>[5x]MYFFSVDPRNGASKSGDVCGSCCCESISARPGEVNGVMVSYAAWSAPLRGHGLTNKTTFEIDGVSVTPPKVSNAFGRTKVGVVFEGTLSDLFPNPEGEQVEYEISELNGPSNGVVELGANGAFTYTPGALFTGVDRFWFSINGNIGEYVISVDPTTSELPQPPFTTPVYVPAARRSVDPRTHVLKFVLGVSPAAIPGDVYRLTVRQVAIDCDGNEFVHISCYDISIGSCG;>METKLTYGNRVTLPEFAKYIVAPAFHEIEGRAIPVTGVDDDASGTQATKLPFVLVGLRQGDTSGPATIAGNSTINLRDDFIVEFNMKKERYRDRKGGETPFFSYYDYESIRDRLFNSMIEFSGEHGITFEFVSLDISTEGDVVYIEFRFRQNYEWCETVREADTTIEAGRFSINLQGC[2x];>MACNKQNGVKNILITFTDCDTQEVIGPISHEQPDDTLPTYKNCAWTNTALTNGYVQRSASNATMTLPVVRDLRVPLAFYQGCAQVDVQVEKFDGTVMTLTEGAVVEPEESDGRSVTMNIVASEIDELLPPGSLAAA[4x];>MAQDALSDGFVRLCIDPSLNFFGEGCKILVEGQMTDDGSATPDAVTCVTSELDIIERFGQGSVLTESLRKVFCTCKSGVSVYALPREDAAAGVKAVYTLTIAGPATTDGRVQLYMGEAEYAVDIGVDAGDTATDIAAAIVAAISPDFPYAATAAAGVITLTARNAGTIGNHLSVIYTNLGSCTSVTPEGVTVTFAQTTAGSVNPTPNDYATVVNECCFAVYVLSSDDTDWQENLRDWIRSAWDCSKPQCFGHGYVFNKGTLGQVLADGDNSAELSRLALPTTYPVLPYLTNAAYGALSACSTCNNPELNIQGQTFGLLSCINMPESCTPGWTFGEVTQLQANGFVVSGPSTTSGQGNYTSPYIYNDVTNYLRDEKNRPNATFRDASSRRLAAATGVALAEFLQQFNGLAVFTKNTNIRTGIIGTNPRLMLGKIRKWAQDNVGTLFSEFDNINEDIQLLTDFEVQPKCVGQPGIFHLNMRYRPPVRGARINVNMAPALFDNCDR[4x]

Caudovirales, the taxonomic order for the tailed double-stranded DNA bacteriophages, is characterized by the presence of a tail—a host cell attachment organelle that is connected to the genome-containing spherical or elongated capsid via a neck. We describe cryo-EM structures of the neck, the neck-capsid and neck-tail junctions, and capsid of the Agrobacterium phage Milano. The tail to capsid junction involves a symmetry mismatch that is bridged by the neck, and is therefore crucial for the assembly of tailed phage. The extensive network of disulfide bonds within and between neck, collar, capsid and tail provides an exceptional structural stability to Milano.

A 3-fold symmetrized map focused at the neck-tail junction was used to understand the interactions between the collar and the tail. Namely, the head-proximal end of the collar interacts with the β-sandwich domain of neck 1 (gp14), while the tail-proximal end of the collar interacts with the tail sheath (gp20). The interaction of the C15-symmetric collar with the C6-symmetric tail sheath is more complex. Five collar subunits (e.g., n, n + 1, n + 2, n + 3, n + 4) comprising the asymmetric unit interact with four tail sheath subunits belonging to the two topmost sheath rings (or layers) that we named Fn, Fn+1, Sn, Sn+1, where F and S denote first and second ring, respectively. The collar subunits n (Cys19), n + 3 (Cys19), and n + 4 (Cys23) form disulfide bonds with tail sheath subunits Sn (Cys467), Sn+1 (Cys467) and Fn+1 (Cys244), respectively, thus linking the collar to the tail sheath by nine (three in each of the three asymmetric units) disulfide bonds. Additionally, the Milano collar connects the sheath to the diaphragm-like structure formed by the neck 1 lumen protrusion loop, allowing for the sheath contraction signal to reach to the genome directly, instead of indirectly through the neck proteins, in preparation for genome release during the attachment to the host cell.> MGMRIGIISVGPGNIMNLYRGVKRASENFEDVSIELVESPRNDLYDLLFIPGVGHFGEGMRRLRENDLIDFVRKHVE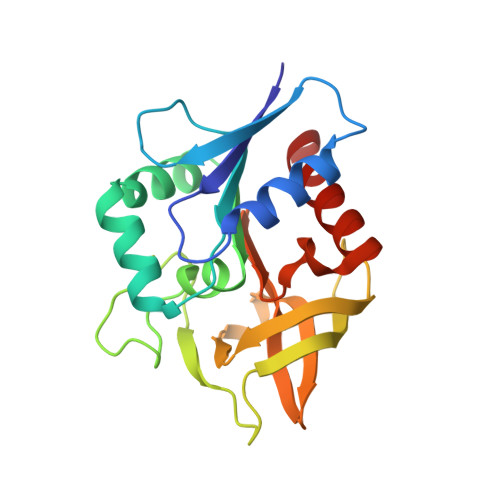DERYVVGVALGMQLLFEESEEAPGVKGLSLIEGNVVKLRSRRLPHMGWNEVIFKDTFPNGYYYFVHTYRAVCEEEHVLGTTEYDGEIFPSAVRKGRILGFQFHPEKSSKIGRKLLEKVIECSLSRR>[8x]MPFHNPFIKDGQIKFPDGSSIVAHVERWAKVRGDKLAYRFLDFSTERDGVPRDLTWAQFSA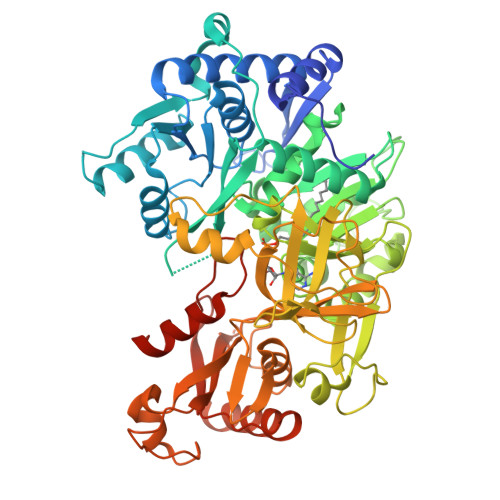RNRAVAARLQQVTQPGDRVAILCPQNLDYLVAFFGALYAGRIAVPLFDPSEPGHVGRLHAVLDNCHPSAILTTTEAAEGVRKFFRTRPANQRPRVIAVDAVPDDVASTWVNPDEPDETTIAYLQYTSGSTRIPTGVQITHLNLATNVVQVIEALEGEEGDRGLSWLPFFHDMGLITALLAPMIGHYFTFMTPAAFVRRPERWIRELARKEGDTGGTISVAPNFAFDHAAARGVPKPGSPPLDLSNVKAVLNGSEPISAATVRRFNEAFGPFGFPPKAIKPSYGLAEATLFVSTTPSAEEPKIITVDRDQLNSGRIVEVDADSPKAVAQASAGKVGIAEWAVIVDAESATELPDGQVGEIWISGQNMGTGYWGKPEESVATFQNILKSRTNPSHAEGATDDATWVRTGDYGAFYDGDLYITGRVKDLVIIDGRNHYPQDLEYSAQEASKAIRTGYVAAFSVPANQLPDEVFENAHSGIKRDPDDTSEQLVIVAERAPGAHKLDIGPITDDIRAAIAVRHGVTVRDVLLTAAGAIPRTSSGKIGRRACRAAYLDGSLRAGKVANDFPDATD>MSNRAKSPALDAVVIGAGVTGIYQAFLINQAGMKVLGIEAGEDVGGTWYWNRYPGCRLDTESYAYGYFALKGIIPEWEWSENFASQPEMLRYVNRAADAMDVRKHYRFNTRVTAARYVENDRLWEVTLDNEEVVTCRFLISATGPLSASRMPDIKGIDSFKGESFHSSRWPTDAEGAPKGVDFTGKRVGVIGTGATGVQIIPIAAETAKELYVFQRTPNWCTPLGNSPMSKEKMDSLRNRYPTILEYVKSTDTAFPYHRDPRKGTDVSESERDAFFEELYRQPGYGIWLSGFRDLLLNKESNKFLADFVAKKIRQRVKDPVVAEKLIPKDHPFGAKRVPMETNYYETYNRDNVHLVDIREAPIQEVTPEGIKTADAAYDLDVIIYATGFDAVTGSLDRIDIRGKDNVRLIDAWAEGPSTYLGLQARGFPNFFTLVGPHNGSTFCNVGVCGGLQAEWVLRMISYMKDNGFTYSEPTQAAENRWTEEVYADFSRTLLAEANAWWVKTTTKPDGSVVRRTLVHVSGGPEYRKRCEQ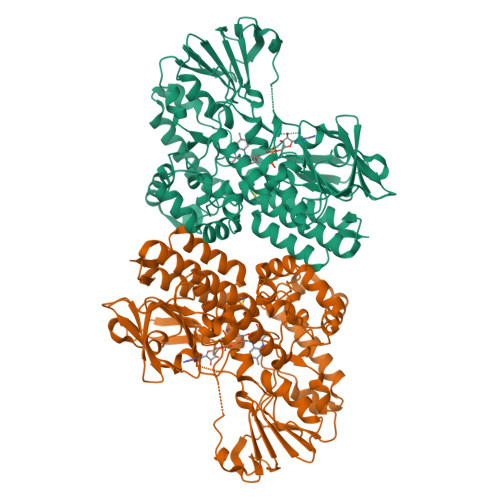VAYNNYNGFELA[2x]> QGTREQLNLCLERLSSGKDKNKSVLQNKYVRCSVRAEVRHLRRVLCHRLMLNPQHVQLLFDNEVLPDHMTMKQIWLSRWFGKPS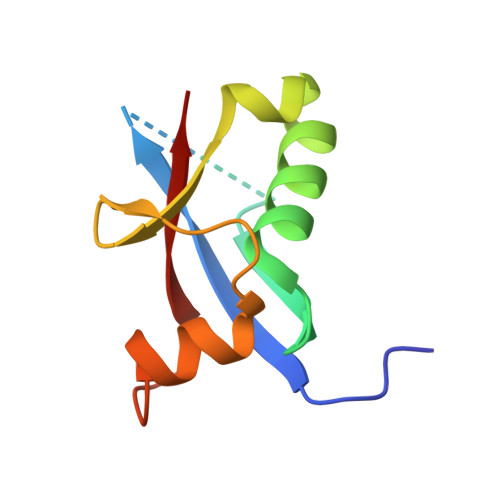PLLLQYSVK1,4,5,6-TETRAHYDRONICOTINAMIDE ADENINE DINUCLEOTIDE PHOSPHATE | C21 H32 N7 O17 P3 | 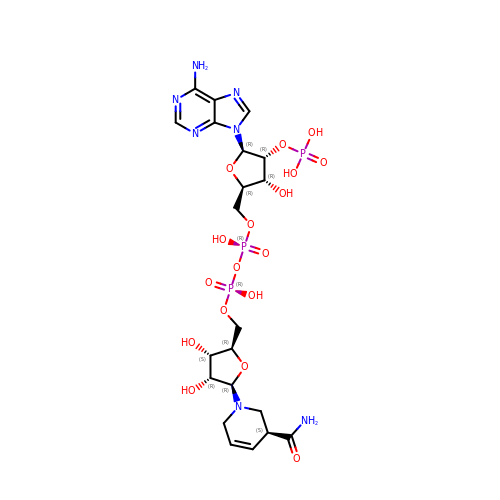MGWIKFWDIJJFDG-ILTSWSAWSA-N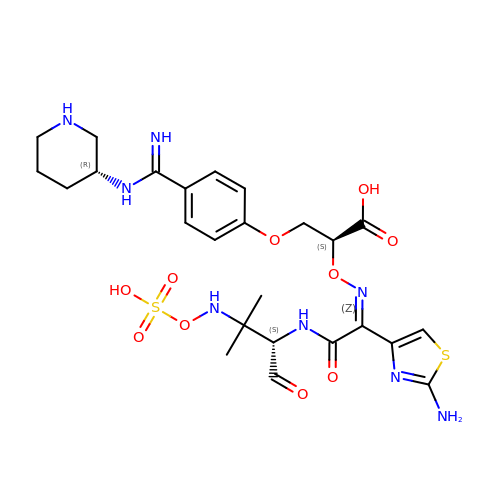(2S)-2-[(Z)-[1-(2-azanyl-1,3-thiazol-4-yl)-2-[[(2S)-3-methyl-1-oxidanylidene-3-(sulfooxyamino)butan-2-yl]amino]-2-oxidanylidene-ethylidene]amino]oxy-3-[4-[N-[(3R)-piperidin-3-yl]carbamimidoyl]phenoxy]propanoic acid | C25 H34 N8 O10 S2 | NFNVPYWCKFTXAX-OOLKDPNPSA-N>[2x]GPLGSRRKFMEFPYVSPTRKQLMVDLMSTVENRLQSQLLPCNLPPDVRNFNNPNGSAEASLHIRSGDKSSPIDFVIGSWIHCKIPTG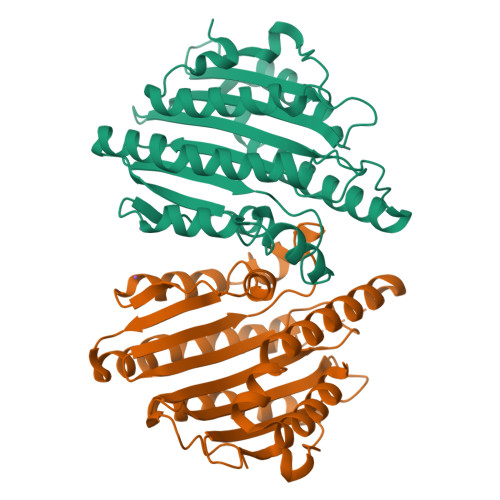VSLNITSISGFLNSSTKAPNFVVELIQSSSKSLVLILDLPHRKDLVLNPDYLKEYYQDTALDSHRQSLLKLPEVNPYVSPSLFVRSAVSPTASMLKIDAEEEDKLEEILRDHVSPAAKEVLEVWLERCVKEEEEKIVVGEEERMELERRDKSFRRKSIEDDLDLQFPRMFGEEVSSRVVHAIKEAFGVL Hsp26 is a small heat shock protein (sHsp) from S. cerevisiae. Its chaperone activity is activated by oligomer dissociation at heat shock temperatures. Hsp26 contains 9 phosphorylation sites in different structural elements. Our analysis of phospho-mimetic mutations shows that phosphorylation activates Hsp26 at permissive temperatures.

Compared to the previous analysis, the new structure revealed that the predominant species of Hsp26 is an oligomer comprising 40 monomers arranged in a raspberry-like shape both for the recombinantly produced proteins and the authentic protein from yeast. We could resolve the structure of the ACD, the CTR, and parts of the MD. Our pseudo-atomic model of Hsp26 consists of residues 63–214 (71% of the sequence). Our structural analysis revealed that the ACDs in Hsp26 adopt the non-metazoan association mode, as the loop containing the β6 sheet can be clearly seen in the density maps and fitting of the wheat ACD domain was possible. These dimers are the principal building blocks of the 40mer. Surprisingly, a β-strand of the MD extends the β-sheet of the ACD and then a helix leads further into the core of the structure. Thus, the MD is intimately connected to the ACD and three MDs associate with each other. While the CTRs exhibit some flexibility, their density is always visible even in asymmetric reconstructions indicating that the IEV motif is predominantly bound to the β4/β8 grove of the adjacent dimer. Based on the 3D structure and the crosslinking data, we suggest an auto-inhibitory locked state in the inactive oligomer where the MD is locked to the loop between the β5 and the β7 strand of the ACD.

>[5x]MSFNSPFFDFFDNINNEVDAFNRLLGEGGLRGYAPRRQLANTPAKDSTGKEVARPNNYAGALYDPRDETLDDWFDNDLSLFPSGFGFPRSVAVPVDILDHDNNYELKVVVPGVKSKKDIDIEYHQNKNQILVSGEIPSTLNEESKDKVKVKESSSGKFKRVITLPDYPGVDADNIKADYANGVLTLTVPKLKPQKDGKNHVKKIEVSSQESWGN4-(3-hydroxyphenyl)-1~{H}-pyrrolo[2,3-b]pyridine-3-carbonitrile 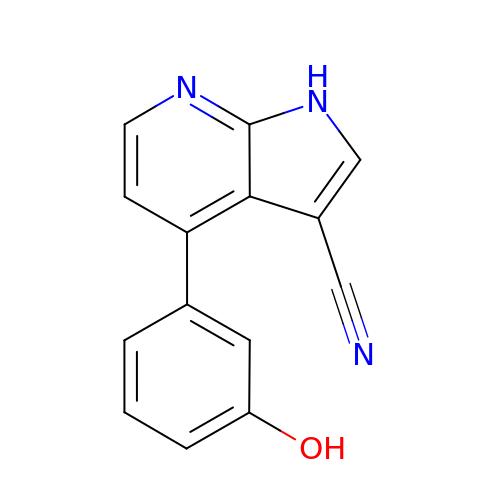| C14 H9 N3 O | NSJGIUMXLVXGPU-UHFFFAOYSA-N>[2x]PLGSVRWARA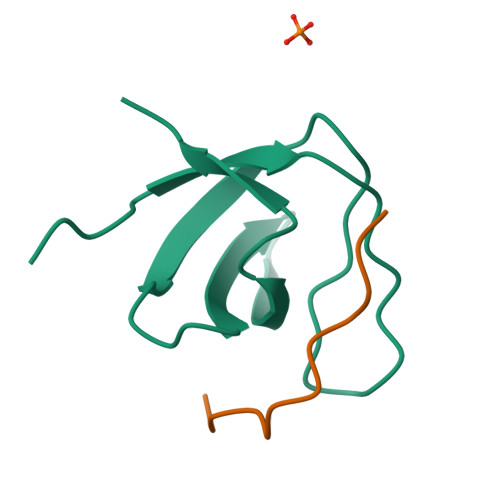LYDFEALEEDELGFRSGEVVEVLDSSNPSWWTGRLHNKLGLFPANYVAPMMR;>PPPRPTAPKPLL[2x]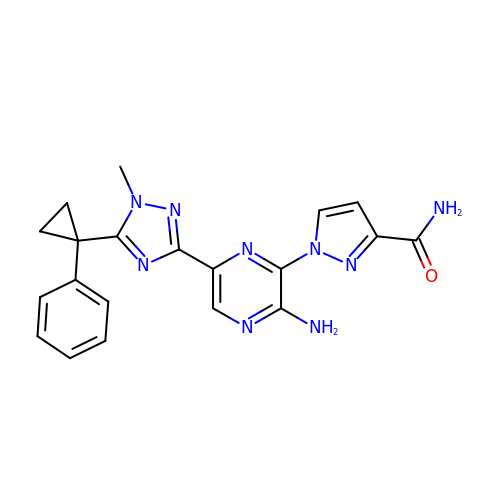1-[3-azanyl-6-[1-methyl-5-(1-phenylcyclopropyl)-1,2,4-triazol-3-yl]pyrazin-2-yl]pyrazole-3-carboxamide | C20 H19 N9 O | PPNTYGOEVAXAOA-UHFFFAOYSA-N>[2x]SNARTGWFSETWR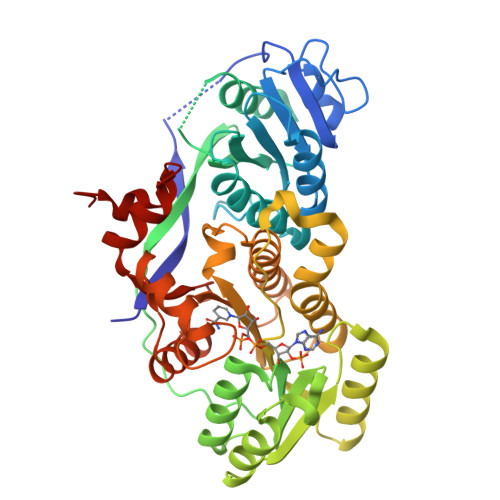QLGRAATADRVPGNWLLLGEVPPALGSLFDDPLTAASWDRSTAPDGVLVGAGAAEDLLAALHEVAGHPTGPVWCVTSRAVGVGTVDDPAADVRAAGVWGLGRVAGLELPDRWGGLVDLPERIDDATRRALAGTLTDDGADDQDGEDQLAVRDGQLWARRLVTTPAPQTGTWTPKGTVLITGGTGGLGGHVARRVAEQGSADRILLLSRQGSAAPGATELLEGIRAFGATAEAVAVDVTDRAAMSGLIDALAAEGAPVRTVVHAAGVVRDVRIAETGAEELAAQMAAKVEGALLLDELLPDLDDFVLFSSISGIWGAAGQAGYAAGNACLDALARRRREQGKRAVSVAWGPWAGGGMLTEHDERELRKRGLTPLLVPAALQAMEQAIMSDRAGDPVVADVTWSRFLPAFTASRPSPLFGSFEEKAA> GAMLKDKSLGEGIKD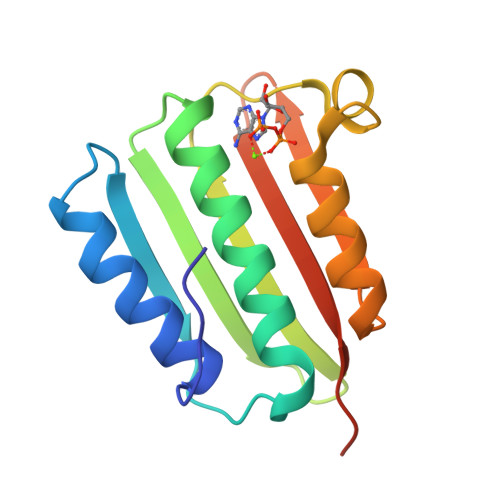LVIDLQKKVPMKVVHEIQDFKVPKGIEDHLFRITQEAISNTLRHSNGTKVTVELFNKDDYLLLRIQDNGKGFNVDEKLEQSYGLKNMRERALEIGATFHIVSLPDSGTRIEVKAPLNKEDSYDD N-{[4-(7H-pyrrolo[2,3-d]pyrimidin-4-yl)phenyl]methyl}benzamide | C20 H16 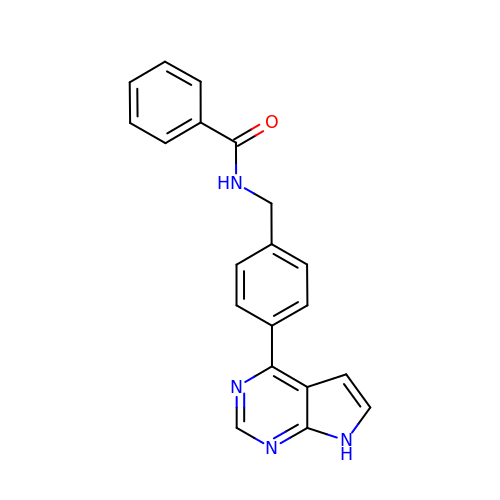N4 O | ZUWTWEPWXCWEFD-UHFFFAOYSA-N>[2x]GAMGGSMSDLDVIRQIEQELGMQLEPVDKLKWYSKGYKLDKDQRVTAIGLYDCGSDTLDRIIQPLESLKSLSELSLSSNQITDISPLASLNSLSMLWLDRNQITDIAPLASLNSLSMLWLFGNKISDIAPLESLKSLTELQLSSNQITDIAPLASLKSLTELSLSGNNISDIA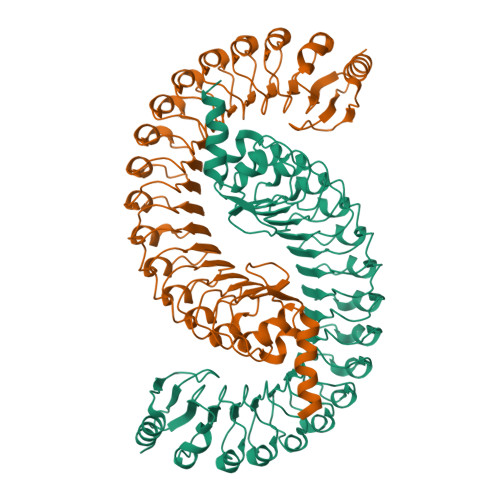PLESLKSLTELSLSSNQITDIAPLASLKSLTELSLSSNQISDIAPLESLKSLTELQLSRNQISDIAPLESLKSLTELQLSSNQITDIAPLASLKSLTELQLSRNQISDIAPLESLNSLSKLWLNGNQITDIAPLASLNSLTELELSSNQITDIAPLASLKSLSTLWLSSNQISDIAPLASLESLSELSLSSNQISDISPLASLNSLTGFDVRRNPIKRLPETITGFDMEILWNDFSSSGFITFFDNPLESPPPEIVKQGKEAVRQYFQSIEEAR>XEVEALEKKVEALELKVQALEK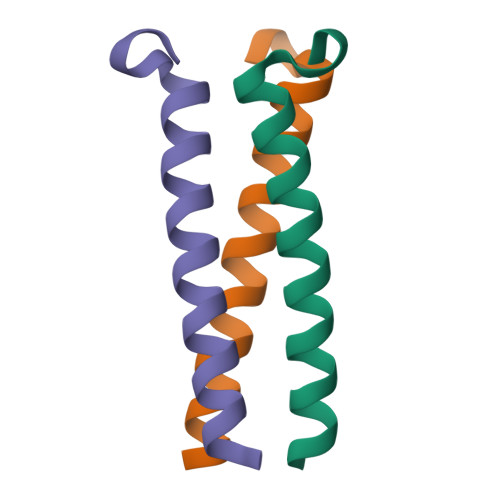KVEALEHGWDGR[2x]> TQFKEIEKTTDFKNHSLPLARIKKIMKADEDVRMISAEAPVVFARACEMFILELTLRSWNHTEENKRRTLQKNDIAAAVTRTDIFDFLVDIVPRGSGSGSGSGSGSDPASQMITVTQLSPMDREARVLRYREKRKTRKFEKTIRY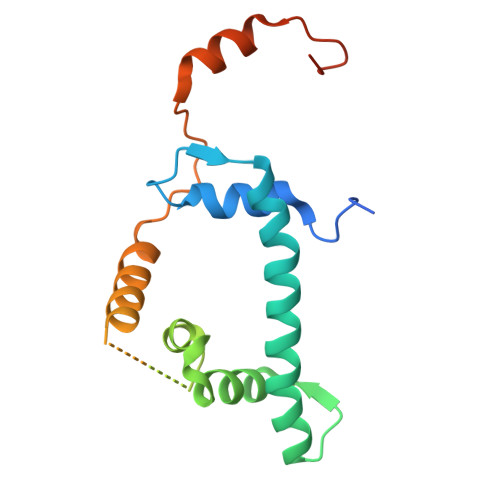ASRKAYAEIRPRVNGRFAKREIEAEEQGF The Q63NT7 protein from Burkholderia pseudomallei is 212 amino acids in length (molecular mass 22.5 kDa). It contains two predicted domains: an N-terminal domain of unknown function (14.5 kDa; DUF1842) and the C-terminal domain (DUF1843; 5.4 kDa), which tends to appear in multiple paralogous copies within individual bacterial operons. The N-terminal domain was predicted to fold into a β-barrel composed of eight antiparallel strands. Polar residues are found covering the exterior surface of the β-barrel, while the interior of the β-barrel is lined with mostly hydrophobic residues, without space for a channel through the barrel.

Q63NT7 presented a challenge for obtaining large, well ordered crystals. We also observed inconsistent crystal formation across our replicated crystal trays. Even so, we were ultimately (after approximately six months) able to optimize these conditions and grow larger rectangular-shaped crystals that diffracted beyond 3 Å resolution on a synchrotron microfocus beamline. We collected data sets from these crystals, which we refer to as form 1. Diffraction data indexing revealed the space group to be P21. The highest resolution resulted from data collected from a single crystal specimen. Efforts to phase the highest quality data set (form 1) using experimental techniques did not lead to immediate success; selenomethionine-labeled protein crystals did not diffract, and we observed no heavy-atom signal in the diffraction patterns of crystals soaked in caesium chloride or potassium iodide. Form 1 crystals gave a combined LLG value of 719, form 2 crystals gave an LLG value of 394 and form 3 crystals gave an LLG value of 305. Because the form 1 crystals gave the highest resolution diffraction data (from X-rays), a model for the β-sheet-rich domain was refined against these data and then subsequently used as the starting point for model refinements of the other crystal forms (X-ray and electron). Final refinement for the form 1 model gave an R factor of 25.1% and an R free of 28.7%. The backbone r.m.s.d. values between the experimental structures and the AlphaFold model were 0.35 Å for form 1, 0.49 Å for form 2 and 0.46 Å for form 3.

>[2x]MSEDLRVGLFPVRYLVGTGLPGAPQLVLDLMVDTVDHSVVGRAAVSQAVSPPLNFHADVWGSYVFRLGPPPRRDGSGAIVQISLQGNQGGPQSNSMITFYGELLLKGDGKTGVASYRYYSNGSWHEVENVPVKADPELVPIEPGPVIGQSSMSAIGSAAMYGVAIQSAAASGDLAHMRTLSAYARQQLESRDEIAAALSELKAEIAKLESRQHHHHHH A conspicuous exception is the interaction of monosialotetrahexosylganglioside (GM1) with the carbohydrate-recognition domain of cholera toxin from Vibrio cholerae: this is one of the strongest protein–carbohydrate interactions known. A conspicuous exception is the interaction of the human ganglioside GM1 with the B subunit pentamer of cholera toxin (CTB5) from Vibrio cholerae, an interaction for which affinities in the range from KD = 4.6 × 10–10 M8a to KD = 5.0 × 10–8 M8b have been reported. The crystal structure of the CTB5-GM1 epitope complex was published in 1994 by Merritt et al. and reveals important H-bonds between the C2 C(sp3)–OH of the terminal galactose and Asn90, Asn14, and a water molecule (right). It is reported that essentially all of the binding energy is due to interactions with this galactose residue and the sialic acid motif.

To establish the importance of a long-discussed key hydrogen bond between C2 of the terminal galactose of GM1 and the B subunit pentamer of cholera toxin (CTB5), the total synthesis of a selectively fluorinated GM1 epitope was conducted in 19 steps. Competition studies have revealed that fluorination of the terminal galactose weakens binding to cholera toxin compared with the natural ligand GM1 but that the binding strength is of the same order of magnitude (about 3 times weaker): this suggests that all other important interactions are preserved. Unexpectedly, the addition of F-GM1, but not GM1, to CTB5 led to severe protein precipitation at protein concentrations required for crystallography. This problem was circumvented by crystallizing the protein with a disaccharide and then exchanging the ligands in situ by carefully timed soaking with high concentrations of F-GM1 (details can be found in the Supporting Information). Crucially, F-GM1 was found to be bound in the same binding mode as GM1 with one crucial difference in the terminal fluorinated galactose unit. The OH → F substitution at C2 of the terminal galactose led to a change in conformation. The quasi-axial arrangement of the C(sp3)–F bond of the d-galactose enables a Dunitz–Diederich-type interaction15a,35 with the adjacent GalNAc C(sp2)=O (3.4 Å). Moreover, this permits an interaction with the side chain residue N90 of the protein (3.6 Å). These interactions abolish the formation of the important hydrogen bonds (CTB5, Asn14, and Asn90; Figure 5C versus Figure 5D) and confirm the working hypothesis.

>TPQNITDLCAEYHNTQIHTLNDKIFSYTESLAGKREMAIITFKNGATFQVEVPGSQHIDSQKKAIERMKDTLRIAYLTEAKVEKLCVWNNKTPHAIAAISMAN[10x]>MGRAHKETLDKLTNAAINKINLLNTSKVKYLVSSAFAGLYVGIGILLIFTIGGLLTDAGSPMTKIVMGLSFAIALSLVIMTGTELFT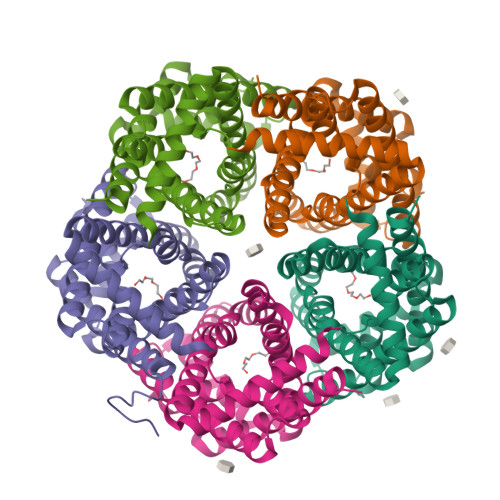GNNMVMSAGMLNKGVSIKDTSKIWAYSWVGNLIGALVLGIIFVGTGLVDKGPVAEFFANTAASKASMPFTALFFRGILCNILVCVSVLCSFRTNSDTAKIIMIFLCLFAFITSGFEHSVANMTIYSVSLFSPTISTVTIGGAIYNLVAVTLGNIVGGALFMGLGTYILGKEKLNAAAENLY[5x]> GSHMEEDALWE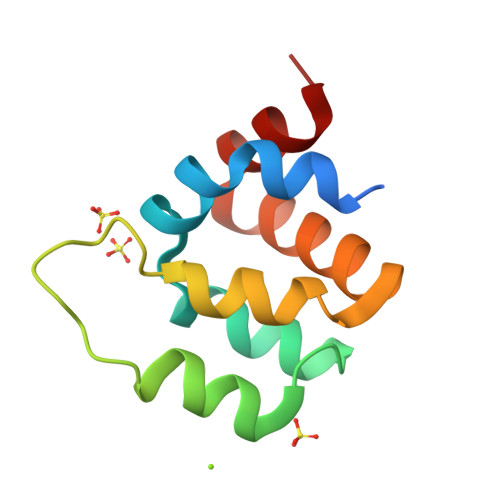NVECNRHMLSRYINPAKLTPYLRQCKVIDEQDEDEVLNAPMLPSKINRAGRLLDILHTKGQRGYVVFLESLEFYYPELYKLVTGKE>[2x]THWFHRNPLKATAPVSFNYYGVVTGPSASKICNDLRSSRARLLELFTDLSCNPEMMKNAADSYFSLLQGFINSLDESTQESKLRYIQNFKWTDTLQGQVPSAQ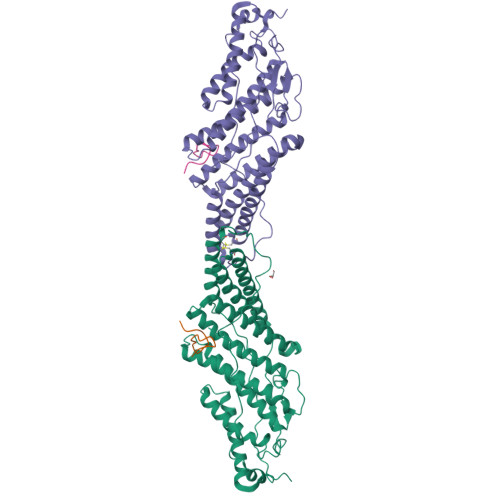QDAVFELISMGFNVALWYTKYASRLAGKENITEDEAKEVHRSLKIAAGIFKHLKESHLPKLITPAEKGRDLESRLIEAYVIQCQAEAQEVTIARAIELKHAPGLIAALAYETANFYQKADHTLSSLEPAYSAKWRKYLHLKMCFYTAYAYCYHGETLLASDKCGEAIRSLQEAEKLYAKAEALCKEYGETKGPGPTVKPSGHLFFRKLGNLVKNTLEKCQRENGFIYFQKIPTEAPQLELKANYGLVEPIPFEFPPTSVQWTPETLAAFDLTK;>RSYGTPELDEDDLEAELDALGDELLADEDSSYLDEAASAPAIPEGVPTDTKNKDGVLVDEFGLPQIPAS[2x]> GVSKEEYKDVETAKKEKEQLGELMEPALGYVVKVPVSSFENKKVDISDIEVITNGNLDDVPYKANSSKYNYPDIKTKDSSLQYVRSGYVIDGEHSGSNEKGYVYYKGNS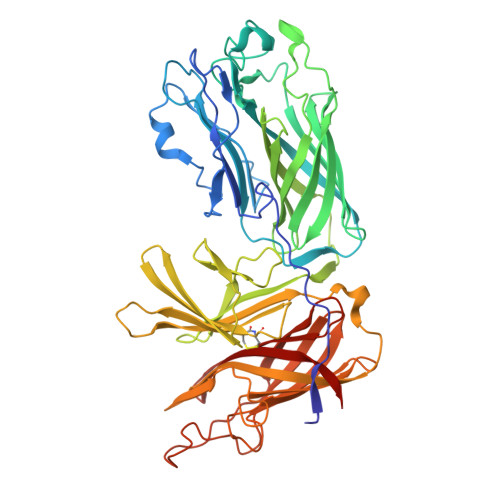PAKELPVNQLLTYTGSWDFTSNANLNNEEGRPNYLNDDYYTKFIGKRVGLVSGDAKPAKHKYTSQFEVDFATKKMTGKLSDKEKTIYTVNADIRGNRFTGAATASDKNKGKGESYNFFSADSQSLEGGFYGPKAEEMAGKFVANDKSLFAVFSAKHNGSNVDTVRIIDASKIDLTNFSISELNNFGDASVLIIDGKKIKLAGSGFTNKHTIEINGKTMVAVACCSNLEYMKFGQLWQQAEGGKPENNSLFLQGERTATDKMPKGGNYKYIGTWDAQVSKENNWVATADDDRKAGYRTEFDVDFGNKNLSGKLFDKNGVNPVFTVDPKIDGNGFTGKAKTSDAGFALDSGSSRYENVKFNDVAVSGGFYGPTAAELGGQFHHKSENGSVGAVFGAKQQVKK> KQKVINVKEVRLSPTIEEHD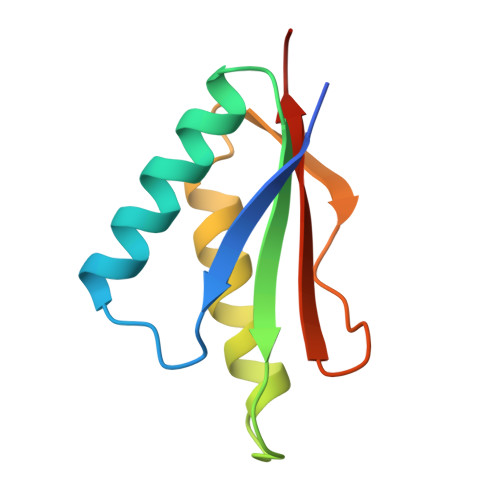FNTKLRNARKFLEKGDKVKATIRFKGRAITHKEIGQRVLDRLSEACADIAVVETAPKMDGRNMFLVLAPKNDNK> MNDIVSAKVLEYKGKKLNFTPEDPAEETIPADELHEHLQKPSTARTKRLKERCRWKHASAGEFIEKSVTAGIERMRYLTEAHKASEGKPEAIRRALGLANVLNKSTLVLQEDEFIVGYHAEDPNMFPLYPELSHMAVQDYLRSDYSPQPADEAAAINEYWKPHSLQSKCQPYFDPADLGRMYQVSSMEAPSFASGYNSIVPPYETVLEDGLLARIKLAEKHIAEAQADMSTFPWNGTKGLDNIAKIDNWKAMVIACKAVISWARRQ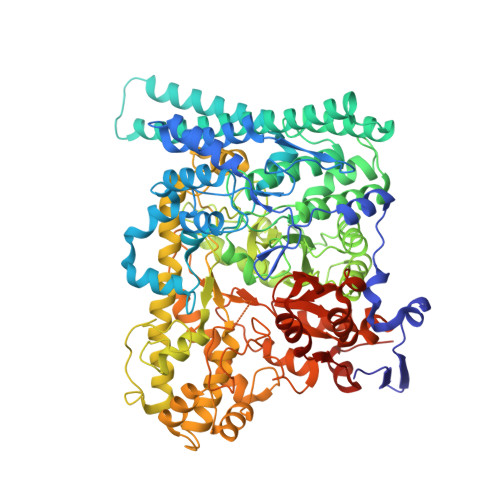GRLCKIVAENFETDPKRQAELLEIADICQRIPAEPCKGLKDAMQAKFFTFLICHAIERYASGYAQKEDTLLWPYYKASVVDKKFQPMSHMDAVELVEMERLKISEHGAGKSRAYREIFPGSNDLFILTVGGTNAKGEDACNDMTDAILEAAKRIRTAEPSIVFRYSKKNREKTLRWVFECIRDGLGYPSIKHDEIGTEQMKEYAKFSLNGNGATDEEAHNWVNVLCMSPGIHGRRKTQKTRSEGGGSIFPAKLLEISLNDGYDWSYADMQLGPKTGDLSSLKSFEDVWEAFRKQYQYAINLCISTKDVSRYFEQRFLQMPFVSAIDDGCMELGMDACALSEQPNGWHNPITTIVAANSLVAIKKLVFEEKKYTLEQLSQALKANWEGFEEMRVDFKRAPKWGNDDDYADGIITRFYEEIIGGEMRKITNYSGGPVMPTGQAVGLYMEVGSRTGPTPDGRFGGEAADDGGISPYMGTDKKGPTAVLRSVSKVQKNQKGNLLNQRLSVPIMRSKHGFEIWNSYIKTWHDLNIDHVQFNVVSTDEMRAAQREPEKHHDLIVRVSGYSARFVDIPTYGQNTIIARQEQDFSASDLEFLNVEISGTGSGSSHHHHHH>MSVSAFNRRWAAVILEALTRHGVRHICIAPGSRSTLLTLAAAENSAFIHHTHFDERGLGHLALGLAKVSKQPVAVIVTSGTAVANLYPALIEAGLTGEKLILLTADRPPELIDCGANQAIRQPGMFASHPTHSISLPRPTQDIPARWLVSTIDHALGTLHAGGVHINCPFAEPLYGEMDDTGLSWQQRLGDWWQDDKPWLREAPRLESEKQRDWFFWRQKRGVVVAGRMSAEEGKKVALWAQTLGWPLIGDVLSQTGQPLPCADLWLGNAKATSELQQAQIVVQLGSSLTGKRLLQWQASCEPEEYWIVDDIEGRLDPAHHRGRRLIANIADWLELHPAEKRQPWCVEIPRLAEQAMQAVIARRDAFGEAQLAHRICDYLPEQGQLFVGNSLVVRLIDALSQLPAGYPVYSNRGASGIDGLLSTAAGVQRASGKPTLAIVGDLSALYDLNALALLRQVSAPLVLIVVNNNGGQIFSLLPTPQSERERFYLMPQNVHFEHAAAMFELKYHRPQNWQELETAFADAWRTPTTTVIEMVVNDTDGAQTLQQLLAQ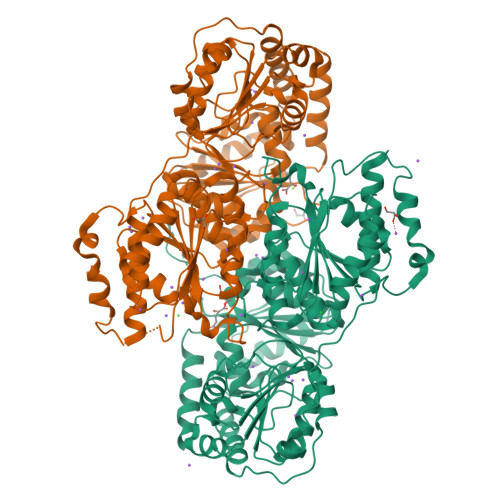VSHL[2x]> MSFVKDFKPQALGDTNLFKPIKIGNNELLHRAVIPPLTRMRALHPGNIPNRDWAVEYYTQRAQRPGTMIITEGAFISPQAGGYDNAPGVWSEEQMVEWTKIFNAIHEKKSFVWVQLAVLGWAAFPDNLARDGLRYDSASDNVFMDAEQEAKAKKANNPQHSLTKDEIKQYIKEYVQAAKNSIAAGADGVEIHSANGYLLNQFLDPHSNTRTDEYGGSIENRARFTLEVVDALVEAIGHEKVGLRLSPYGVFNSMSGGAETGIVAQYAYVAGELEKRAKAGKRLAFVHLVEPRVTNPFLTEGEGEYEGGSNDFVY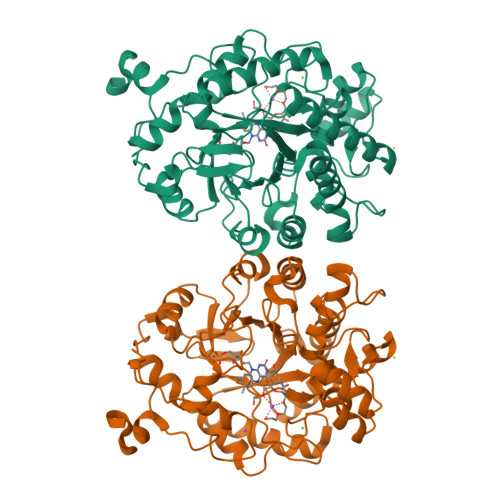SIWKGPVIRAGNFALHPEVVREEVKDKRTLIGYGRFFISNPDLVDRLEKGLPLNKYDRDTFYQMSAHGYIDYPTYEEALKLGWDKK> GMALTPDQMPDRAEVVFTCNGKAVGKMRNELDVAMVKPFEERFALATDEGAFHGGDASAPPPLALFIAGLTGCVMTQIRAFAKRLKVTVTDLDVECRVVWDWAKAGPVYETGPKSFEIDIILHSPDPIEAQQALI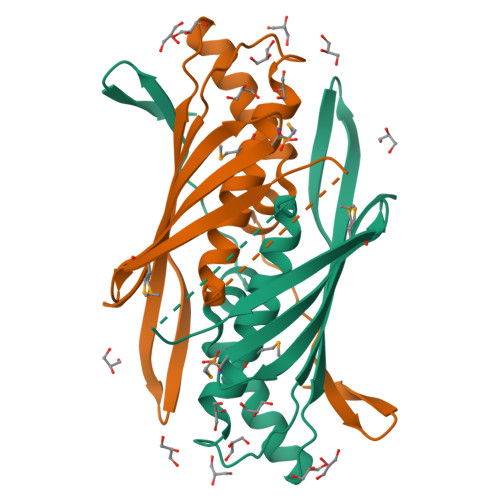EAAKKGCFLEQTLGQANTIRHRLKVGDTFIDA> GSEFPLDTSLRLKTFSSKSEYQLVVNAVRKLQESGFYWSAVTGGEANLLLSAEPAGTFLIRDSSDQRHFFTLSVKTQSGTKNLRIQCEGGSFSLQSDPRSTQPVPRFDCVLKLVHHYMPPQALPGSTPKRAYYIYSGGEKIPLV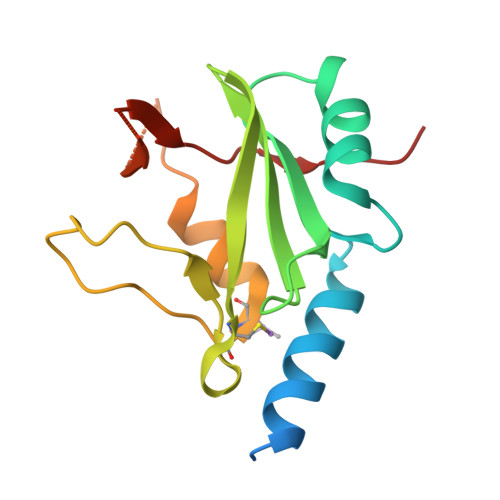LSRPLSSN>MGSDKIHHHHHHMEDGMNTFDLYYWPVPFRGQLIRGILAHCGCSWDEHDVDAIEGLMDCGAEKQPVAFMGPPVLIDRERNFAISQMPAIAIYLGERLDILPATVEGRTLSAKIVNDANDVLDELTLNGGREMWTPEKWQEFVPRLQKWI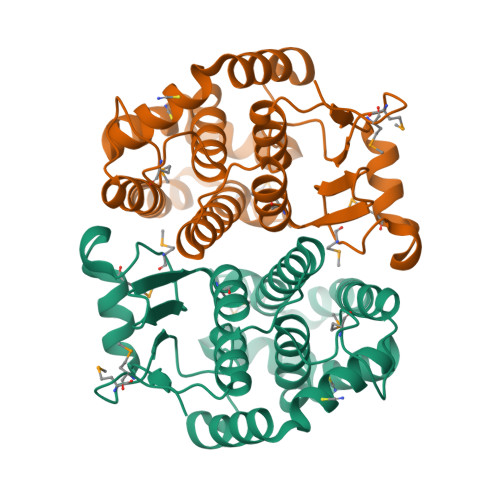RIFADTGARNGLSAASGFMLGTEKIGVADIVTAILWTTVADRFPAIKGIIEDTSPIIWGLSRRVVATAPLAALNSKSFEEYGNAYCGGEIEKSLRKVAS[2x]> MNRIPAATRNAPMYATAMSQFAVCRQPWNEYISLLTKDDAQPFHTTPQEKPAYRGRKRGREGWLFGQQ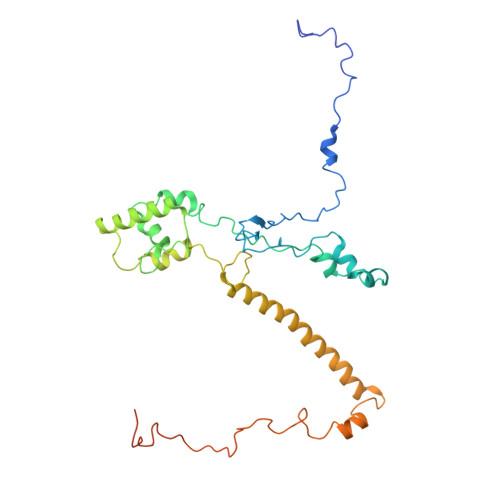VQLHYHRFPDEQLFTNLTRWRMGDTVGDVAIQQFRNAQPFDIEDKDPQGFQRPAPEVYMKLNYKNPATISRFLTRTGHMYPQDIMPLNPEAVVKLRVAKAQAIRIGLYPRFGNPFWFRSQSFRPKAYQENYDPTTYSTKHTMEHFAYNWVQTDRIRQYFKGLEELHQSRRATASSGGGGVTSEHKQQSQLYALDNMSIEMHRNAPSYRADVERSIKKPTVPGLMSTKGMKKKFHNLYSSTSTKRMGFSNPTLGIKKV>[16x]MSQQPGVLPENMKRYMGRDAQRMNILAGRIIAETVRSTLGPKGMDKMLVDDLGDVVVTNDGVTILREMSVEHPAAKMLIEVAKTQEKEVGDGTTTAVVVAGELLRKAEELLDQNVHPTIVVKGYQAAAQKAQELLKTIACEVGAQDKEILTKIAMTSITGKGAEKAKEKLAEIIVEAVSAVVDDEGKVDKDLIKIEKKSGASIDDTELIKGVLVDKERVSAQMPKKVTDAKIALLNCAIEETASEMLKDMVAEIKASGANVLFCQKGIDDLAQHYLAKEGIVAARRVKKSDMEKLA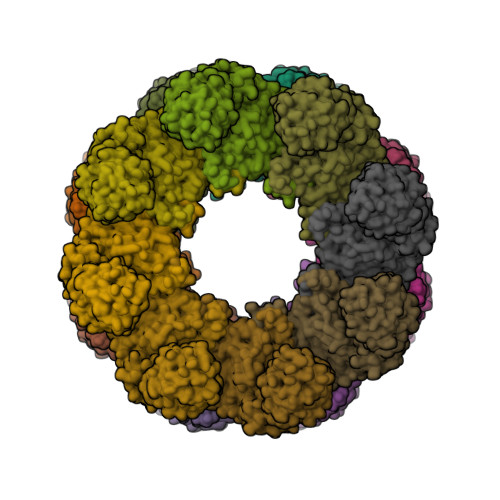KATGANVITNIKDLSAQDLGDAGLVEERKISGDSMIFVEECKHPKAVTMLIRGTTEHVIEEVARAVDDAVGVVGCTIEDGRIVSGGGSTEVELSMKLREYAEGISGREQLAVRAFADALEVIPRTLAENAGLDAIEILVKVRAAHASNGNKCAGLNVFTGAVEDMCENGVVEPLRVKTQAIQSAAESTEMLLRIDDVIAAEKLRGAPDMGDMGGMPGMGGMPGMM hypochlorous acid | Cl H O | 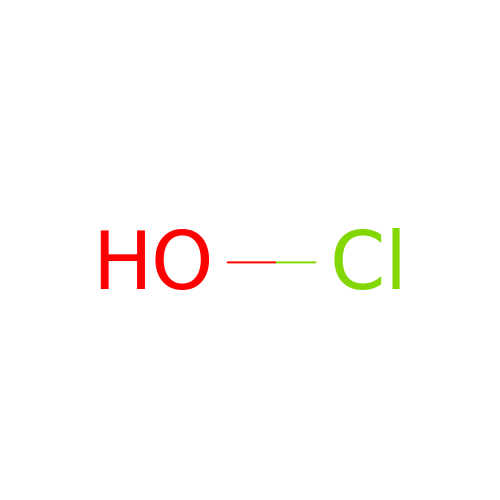QWPPOHNGKGFGJK-UHFFFAOYSA-N> SNALFGVTSELSKDGRERIYRVEGQLFYASVEDFMAAFDFREALDRVVIDVSRAHIWDISSVQALDMAVLKFRREGAEV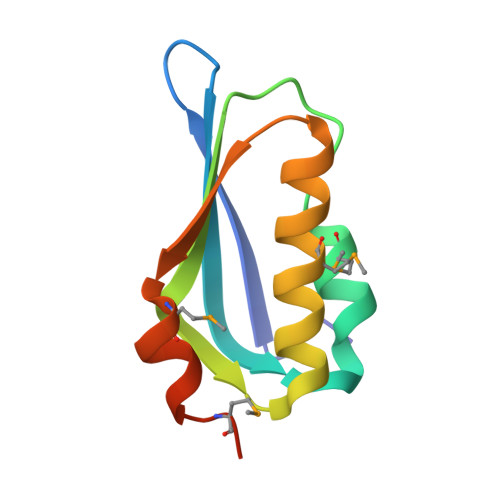RIVGMNEASETMVDRLAIHD> MGHHHHHHHHHHSSGHIEGRHGENLYFQGMRYRQVHLDFHTSEHISDIGRNFSKKNFQEMLQLGHVNSITVFAKCHHGWAYFPSATNEIHPRLDFDLLGAQIEAAHEIGVKVPIYISVGFDEKLAWEKPQWLMRDEADRMNWVDSFMKPGYHQFCLNTPYLDLVIEQVQEVVRKYDGDGIFLDIVGERTCYCTTCLKQMQADGLDPHNKEDVIANGRRIYANYTTRIREAIDAIKPGLPVFHNAGHIHQGRRDLMGMNSHLELESLPTGGWGYDHFPLSARYAQPTGFHFLGMTGKFHTFWGEFGGYKHPNALRYETALSLANGARCSIGDQLHPGGQMDRATYELIGKAYAEVEAKEAWCVNAVNLADVALLTVEAAGVQQESGAMYSGKVDMGAVRMLLEGKILFDIVDLESDWSGYKVLILPDSIVMKDTILPKVEAFLAAGGKVLASGRSGLNVELTRQMLPLGFTDSGLNPFRPDYFRPLCDGMANLGEAAYVMYGDGRRIELTDGTELGRREDPYFNRQAFRFCSHQHAPSSEQEGGPGMVESAQGIYIAWNVFE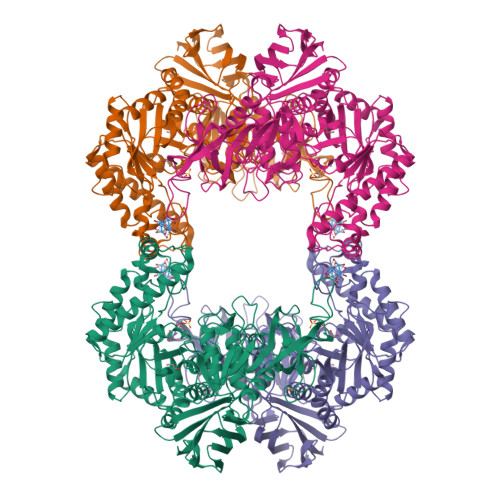DYATKGSLILKEMVLFALRRLLGEQITLKTTLPAQGVTTLQHQAAERRYINHLLYASPVKRGERVEIIEDMIPLQQVEVQLQLPVTDVKRVYLAPQMTEIEFKASGGDVQFTVPQLECHQMVVVEYNE> MCQM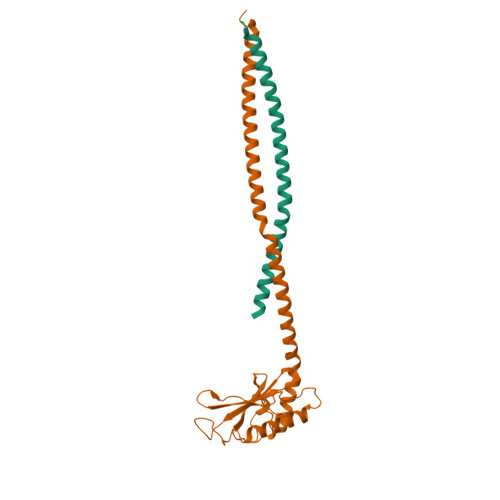TKNKYATVDFDQVNEKGLKSLITAINKTGVTVIEVDSSNRATTKDGVKVKTAKLVLSDGQILAIQVNDTGDISSVKLNGKAIPNAQSPDIKTLGTVMGQAARKNSAKFQKSLIAKAKRVANPVDKKPAVKSNFQRLQEAKQRNAQVVAAYKSAQNSVSFNQQQITDLRAKLDKETGRLNNEKARNGELKRRLKQLKAGN;> MEQFNINKGMTIKPGLDVLPPPVTDDEYRALMAGEDRYLMTESNTLEEIEATFFYDTPIHWCATDLLEAISSTRLQLHRTMQAFVRALNQKLNGTGISAGSDKTGDVAQSGARAIGGAEIGRARNVNGLPVLPAIIPLSDGQTISILFHSPTAENRITNSDTLVAFQFLLNKKDVTHTVAPMSGRDMTLAQVTMKLANLAEKNSAKFQRAQKKKKALVDEITQLQADSDQKEDAMSDLADQVAAVEGQKADLEQKINAVASEADSLYEENERLQGEIDRLNRTGGRDTIAPAGMTGGHSRALTDRLASIKNRMHMDGEATLSNGASMKQFIGDGEGYIQLTDPDGSVYMIKAKSIQGVDMADAIGKLFKAYKAGNVSEYLVQPEEHKPENVEPESAEDTGSSSPEPEVSVGAYRYALQMRPAAPGAIPEGNKAILPRPDEGDPYYEYARYGIATYDTPLSDQQMSEYDLKLLPREDSFDFLAKTLTNGPFGKYAQKALELATNSPDEFRVMLKTQFQKTFPNIAFPGGAGTEKMVQSMINALQAEVGEITQPEPAPAQPDETVSEADAEANKAIEYLNNVMDMQSTDMAEIRNARGNVREAIAALQTAGRFEENEELVNGAARHLADLLVAIQKAGVAA> G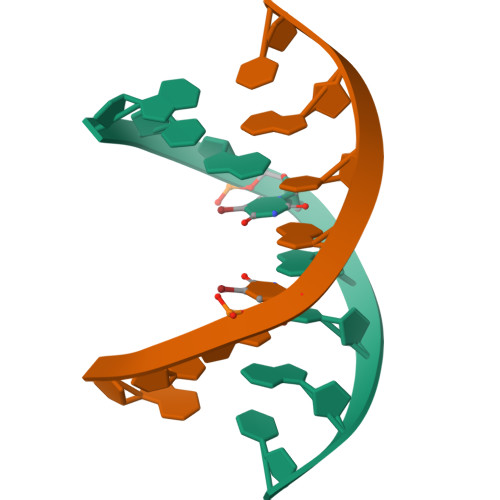TGUACAC> MISLNGYGRFGLQYVEDRGVGLEDTIISSRLRINIVGTTETDQGVTFGAKLRMQWDDGDAFAGTAGNAAQFWTSYNGVTVSVGNVDTAFDSVALTYDSEMGYEWSSFGDAQSSFFAYNSKYDASGALDNYNGIAVTYSISGVNLYLSYVDPDQTVDSSLVTEEFGIAADWSNDMISLAAAYTTDAGGIVDNDIAFVGAAYKFNDAGTVGLNWYDNGLSTAGDQVTLYGNY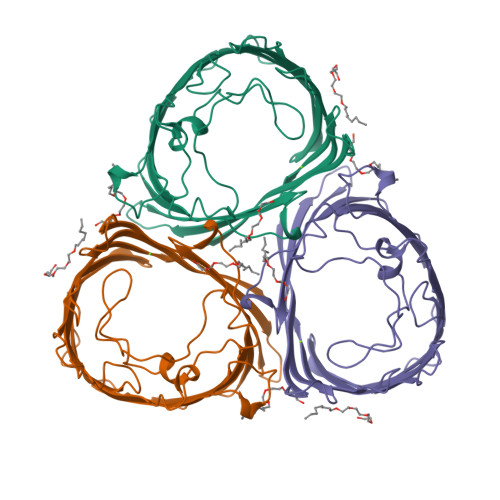AFGATTVRAYVSDIDRAGADTAYGIGADYQFAEGVKVSGSVQSGFANETVADVGVRFDF> YIATRENCCILDERFGSYCPTTCGIADFFNK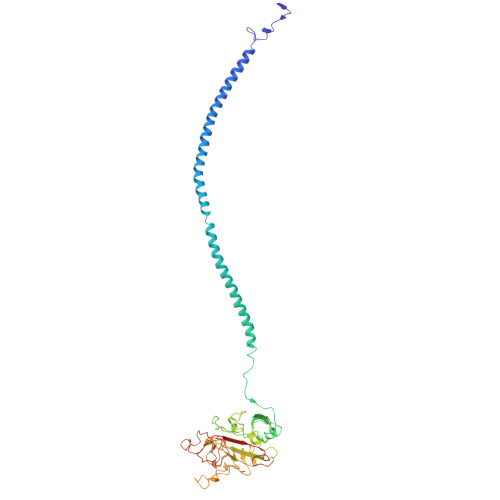YRLTTDGELLEIEGLLQQATNSTGSIEYLIQHIKTIYPSEKQTLPQSIEQLTQKSKKIIEEIIRYENTILAHENTIQQLTDMHIMNSNKITQLKQKIAQLESHCQEPCKDTAEIQETTGRDCQDIANKGARKSGLYFIKPQKAKQSFLVYCEIDTYGNGWTVLQRRLDGSEDFRRNWVQYKEGFGHLSPDDTTEFWLGNEKIHLITTQSTLPYALRIELEDWSGKKGTADYAVFKVGTEEDKYRLTYAYFIGGERGDAFDGFNFGDDPSDKSYTYHNGMRFSTFDNDNDNFEGNCAEQDGSGWWMNRCHAGHLNGPYYIGGVYSRDTGTNSYDNGIIWATWRDRWYSMKKTTMKIIPFNRLSIDGQQHSGGLKQVGDS The ykkC riboswitches comprise a group of three structurally unrelated riboswitches that bind guanidine. The guanidine-II riboswitch comprises two stem–loops with G+C-rich helices and an ACGR (R = A or G) tetraloop, connected by a short polynucleotide of ∼14 nt. Using X-ray crystallography, our laboratory and that of Strobel showed that the stem–loops dimerize by loop–loop interaction involving the formation of intermolecular base pairs and triples. Formation of the dimer creates identical binding sites for two guanidine ligands symmetrically.

For clarity, we term these species diguanidine-C4 [N,N′-(butane-1,4-diyl)bis guanidinium, also known as arcaine] and diguanidine-C5 [N,N′-(pentane-1,5-diyl)bis guanidinium also known as audouine] respectively. Our chemically synthesized diguanidine-C4 was soaked into the G. violaceous P1 stem–loop crystals, and the resulting crystals diffracted to 1.66 Å. The electron density for the C4 linker region is weaker compared to the guanidine groups. Moreover the crystallographic B-factors for these atoms are significantly higher (average value of 57.5) compared to those of the guanidino-C atoms (46.2). These data collectively suggest a greater flexibility of the C4 chain, most likely in a kind of crankshaft rotation. The guanidine groups of diguanidine-C5 and ethylguanidine are within 0.2 Å, but those of diguanidine-C4 are retracted by 0.4 Å. This indicates that the shorter linker may be under some degree of tension. Diguanidine-C4 has a slightly higher affinity than that of diguanidine-C5, most probably because of the greater flexibility of the linking chain in the latter.

> GGUGGGGACGACCCCACC>MSPGSVVVTGANRGIGLGLVQQLVKDKNIRHIIATARDVEKATELKSIKDSRVHVLPLTVTCDKSLDTFVSKVGEIVGSDGLSLLINNAGVLLSYGTNTEPNRAVIAEQLDVNTTSVVLLTQKLLPLLKNAAS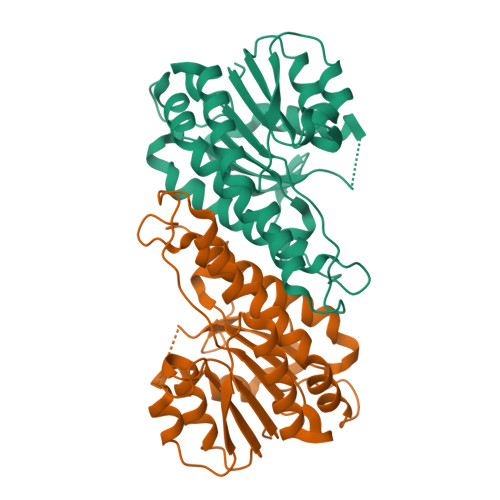KESGDQLSVSRAAVITISSGLGSITDNTSGSAQFPVLAYRMSKAAINMFGRTLAVDLKDDNVLVVNFCPGWVQTNLGGKNAALTVEQSTAELISSFNKLDNSHNGRFFMRNLKPYEF[6x]> 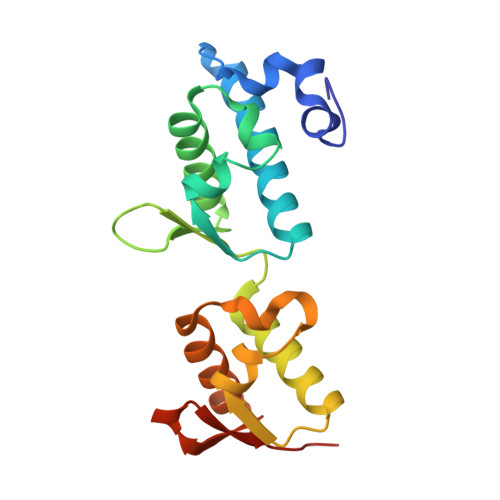MLTVGFEWAAQPEKYPWMYSLPSKTEDFEDWLNQWSDFTLQWFKINKLHQISLVELMGEKPFSYLQNKSKALTVIVENLIARNFCKYTDKEYKSIRVFWRGYRDWSEVIYNWALKKGRTELTFFEIIDLKESPDNFHMLPKEDFKKIFNILVKNKRAEWINKKNMHIRILFLEHHHHHH>[8x]MALVTVPTATTRLRNFCVFSSVKPLDFCDQYSSPCSSDATVDDGWFVCEYHASRFFKMEKLALAIPDGTGNNYYRTVGKSLVDDKAEGIERILIPSQNNYETVLNLSLLGPAERLVFYMIY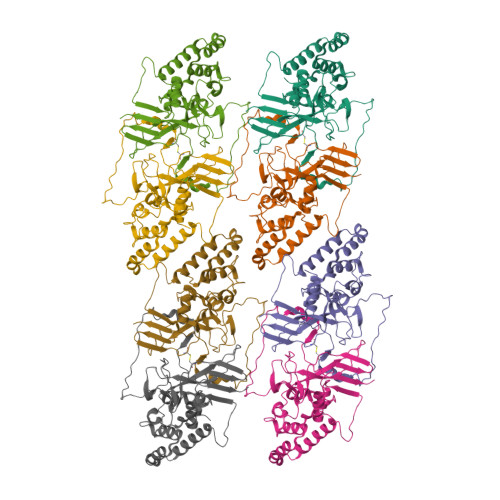DNKEKQNEICQQLRMYERFRPEVVEELYNSTLRVLALTNPDAYCAQTNTNESRSFGLSVEDDLAFNVLPTFIQNLIRKCVAPESLTIGTEDLQLRNCNTCRITSEGLLASVRLYNSVQPKYLYGVNENRLQIRNVLQFQGNANALQQKLSRYELYQINIPLFLGKQIISTGR> PAQDNSRFVIRDRNWHPKALTPDYKTSIARSPRQALVSIPQSISETTGPNFSHLGFGAHDHDLLLNFNNGGLPIGERIIVAGRVVDQYGKPVPNTLVEMWQ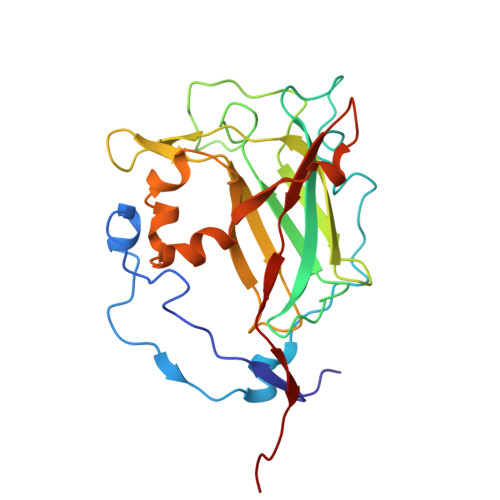ANAGGRYRHKNDRYLAPLDPNFGGVGRCLTDSDGYYSFRTIKPGPAPWRNGPNDWRPAHIYFGISGPSIATKLITQLYFEGDPLIPMCPIVKSIANPEAVQQLIAKLDMNNANPMDCLAYRFDIVLRGQRKTHFENC3-(2-fluorophenyl)-2-methyl-N-((2-oxo-2,3-dihydro-1H-benzo[d]imidazol-5-yl)methyl)acrylamide | C18 H16 F N3 O2 | 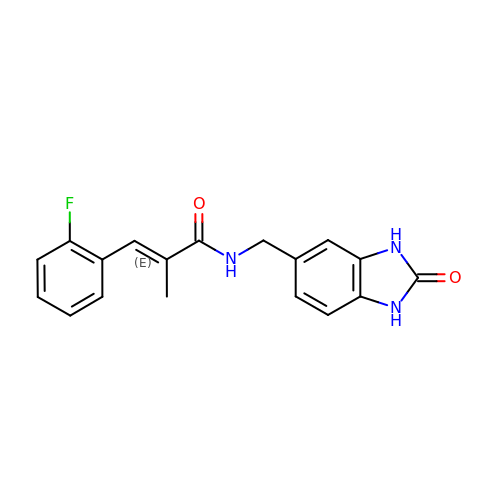MNPHMLQQNDWSRS-DHZHZOJOSA-N> GLVPRGSHMTGRMLTLDGNPAANWLNNARTKWSASRADVVLSYQQNNGGWPKNLDYNSVGNGGGGNESGTIANGATITEMVFLAEVYKSGGNTKYRDAVRKAANFLVNSQYSTGALPQFYPLKGGYSDHATFNDNGMAYA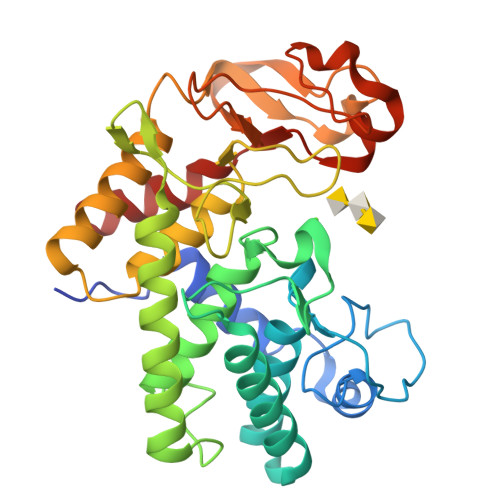LTVLDFAANKRAPFDTDVFSDNDRTRFKTAVTKGTDYILKAQWKQNGVLTVWCAQHGALDYQPKKARAYELESLSGSESVGVLAFLMTQPQTAEIEQAVRAGVAWFNSPRTYLEGYTYDSSLAATNPIVPRAGSKMWYRFYDLNTNRGFFSDRDGSKFYDITQMSLERRTGYSWGGNYGTSIINFAQKVGYL> SNSADE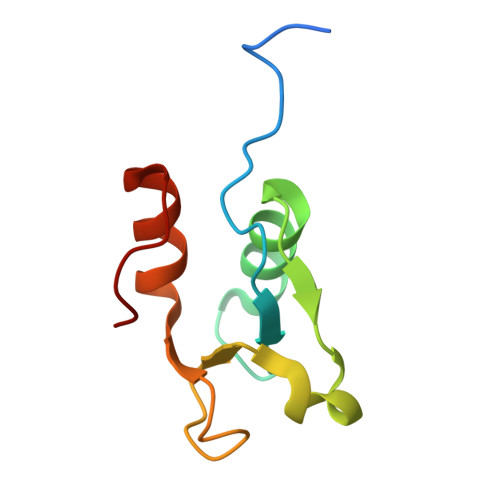TLCQTKVLLDIFTGVRLYLPPSTPDFSRLRRYFVAFDGDLVQEFDMTSATHVLGSRDKNPAAQQVSPEWIWACIRKRRLVAPS>MFSGIKGPNPSDLKGPELRILIVHARWNLQAIEPLVKGAVETMIEKHDVKLENIDIESVPGSWELPQGIRASIARNTYDAVIGIGVLIKGSTMHFEYISEAVVHGLMRVGLDSGVPVILGLLTVLNEEQALYRAGLNGGHNHGNDWG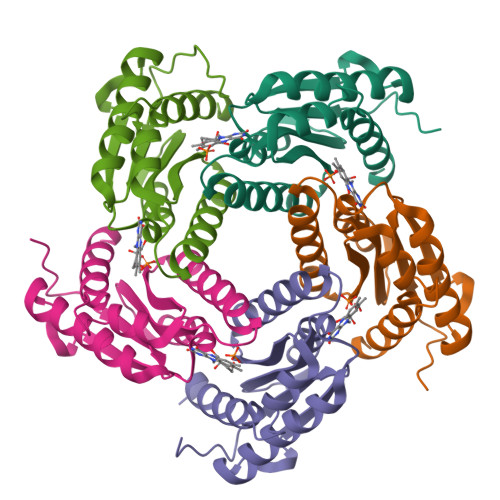SAAVEMGLKALY[5x]uridine-5'-diphosphate-3-O-(R-3-hydroxydecanoyl)-N-acetyl-D-glucosamine 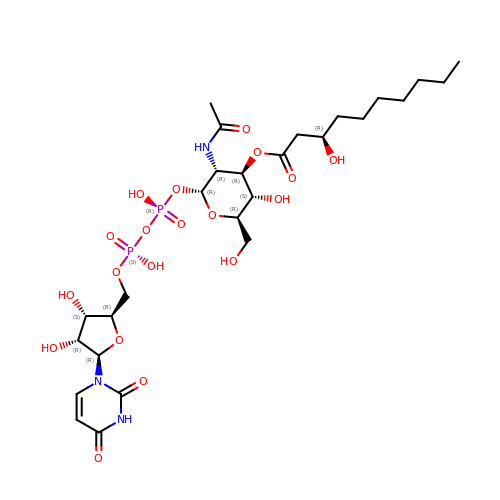| C27 H45 N3 O19 P2 | MQPZMQHQQMJGDE-MCDYFTFASA-N> MSKRIALFPALLLALLVIVATALTWMNFSQALPRSQWAQAAWSPNINVIEQMIFHYSLLPRLAISLLVGAGLGLVGVLFQQVLRNPLAEPTTLGVATGAQLGITVTTLWAIPGAMASQFAALAGACVVGLIVFGVAWGKRLSPVTLILAGLVVSLYCGAINQLLVIFHHDQLQSMFLWSTGTLTQTDWGGVERLWPQLLGGVMLTLLLLRPLTLMGLDDGVARNLGLALSLARLAALSLAIVISALLVNAVGIIGFIGLFAPLLAKMLGARRLLPRLMLASLIGALILWLSDQIILWLTRVWMEVSTGSVTALIGAPLLLWLLPRLRSISAPDMKVNDRVATERQHVLAFALAGGVLLLMAVVVALSFGRDAHGWTWASGALLDDLMPWRWPRIMAALFAGVMLAVAGCIIQRLTGNPMASPEVLGISSGAAFGVVLMLFLVPGNAFGWLLPAGSLGAAVTLLIIMIAAGRGGFSPHRMLLAGMALSTAFTMLLMMLQASGDPRMAQVLTWISGSTYNATDAQVWRTGIVMVILLAITPLCRRWLTILPLGGDTARAVGMALTPTRIALLLLAACLTATATMTIGPLSFVGLMAPHIARMMGFRRTMPHIVISALVGGLLLVFADWCGRMVLFPFQIPAGLLSTFIGAPYFIYLLRKQSRHHHHHHHH;>[2x]MQEYTNHSDTTFALRNISFRVPGRTLLHPLSLTFPAGKVTGLIGHNGSGKSTLLKMLGRHQPPSEGEILLDAQPLESWSSKAFARKVAYLPQQLPPAEGMTVRELVAIGRYPWHGALGRFGAADREKVEEAISLVGLKPLAHRLVDSLSGGERQRAWIAMLVAQDSRCLLLDEPTSALDIAHQVDVLSLVHRLSQERGLTVIAVLHDINMAARYCDYLVALRGGEMIAQGTPAEIMRGETLEMIYGIPMGILPHPAGAAPVSFVY;> MSGLPLISRRRLLTAMALSPLLWQMNTAHAAAIDPNRIVALEWLPVELLLALGIVPYGVADTINYRLWVSEPPLPDSVIDVGLRTEPNLELLTTMRPSFMVWSAGYGPSPEMLARIAPGRGFNFSDGKQPLAMARKSLTEMADLLNLQSAAETHLAQYEDFIRSMKPRFVKRGARPLLLTTLIDPRHMLVFGPNSLFQEILDEYGIPNAWQGETNFWGSTAVSIDRLAAYKDVDVLCFDHDNSKDMDALMATPLWQAMPFVRAGRFQRVPAVWFYGATLSAMHFVRVLDNAIGGKA

As one of the most elegant biological processes developed in bacteria, the siderophore-mediated iron uptake demands the action of specific ATP-binding cassette (ABC) importers. In the periplasm, a group of soluble proteins named periplasmic substrate-binding proteins (SBP) are generally responsible for binding the siderophore-Fe3+ molecules and delivering them to corresponding inner membrane importers. In this study, we functionally characterized the ferrichrome, a hydroxamate-type siderophore molecule, importer FhuCDB complex from E. coli and determined its structure at 3.4 Å resolution by single-particle cryo-electron microscopy (cryo-EM).

To understand the molecular basis of this importer, we determined the structure of FhuCDB in LMNG by single-particle cryo-EM at 3.4 Å resolution. The overall size of the complex was ~130 × 100 × 80 Å3, with one FhuD on the periplasmic side, one FhuB in the membrane, and two FhuC on the cytosolic side. However, a unique feature in FhuCDB was the single membrane subunit of FhuB, comparing to two subunits of homodimers in other known subfamily members. FhuB had 20 transmembrane helices (TM) folding into two domains: N-half with the first ten TMs and C-half with the last ten TMs. In between the two halves, there was a central translocation pathway. Based on a tunnel calculation using the MoleOnline server, the FhuB central pathway was open to the cytosolic side and closed to the periplasmic side, indicating an inward-open conformation. The movement of these residues effectively deformed the original substrate-binding pocket in FhuD and allowed it to be occupied by two loops from FhuB: L5 in between TM5 and H5a as well as L15 in between TM15 and H15a. In FhuCDB, three residues in L5 (F167, D170, Q171) were directly interacting with FhuD residues (N64, W68) via hydrogen bonding. Specifically, these four residues: V165, F176 on the N-half and their counterparts Q498, L509 on the C-half, defined the narrowest position in the pathway, which was then directly closed on top by H169 and M505. Below the periplasmic gate, residues along the path could be grouped into three types: hydrophobic residues with mostly small side chains (A96, G150, L151, L155, G158, A159, L494, I512), polar residues (T91, T92, T97, Q100, S154, N161, Q162, S179, S421, E423, S487, T488, T491, S513) capable of forming hydrogen bonds, as well as Met residues (M175, M495, M492, M484).> LKESPSGYLRSGEGDTGCGELVWVGEPLTLRTAETITGKYGVWMRDPKPTYPYTQETTWRIDTVGTDVRQVFEYDLISQFMQGYPSKVHILPRPLESTGAVVYSGSLYFQGAESRTVIRYELNTETVKAEKEIPGAGYHGQFPYSWGGYTDIDLAVDEAGLWVIYSTDEAKGAIVLSKLNPENLELEQTWETNIRKQSVAEAFIICGTLYTVSSYTSADATVNFAYDTGTGISKTLTIPFKNRYKYSSMIKYNPLEKKLFAWDNLNM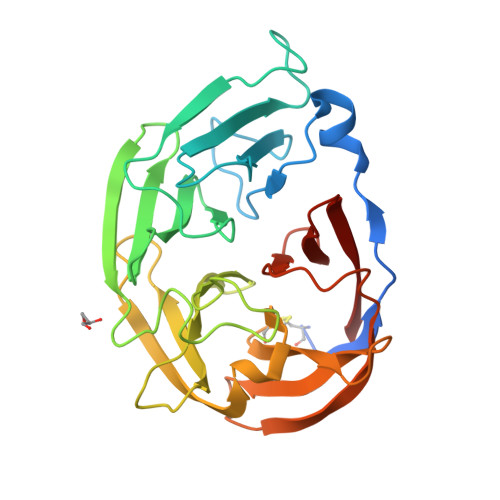VTYDIKLSKM>[8x]SRPLSDQEKRKQISVRGLAGVENVTELKKNFNRHLHFTLVKDRNVATPRDYYFALAHTVRDHLVGRWIRTQQHYYEKDPKRIYYLSLEFYMGRTLQNTMVNLALENACDEATYQLGLDMEELEEIEEDAGLGNGGLGRLAACFLDSMATLGLAAYGYGIRYEFGIFNQKICGGWQMEEADDWLRYGNPWEKARPEFTLPVHFYGRVEHTSQGAKWVDTQVVLAMPYDTPVPGYRNNVVNTMRLWSAKAPNDFNLKDFNVGGYIQAVLDRNLAENISRVLYPNDNFFEGKELRLKQEYFVVAATLQDIIRRFKSSKFGCRDPVRTNFDAFPDKVAIQLNDTHPSLAIPELMRVLVDLERLDWDKAWEVTVKTCAYTNHTVLPEALERWPVHLLETLLPRHLQIIYEINQRFLNRVAAAFPGDVDRLRRMSLVEEGAVKRINMAHLCIAGSHAVNGVARIHSEILKKTIFKDFYELEPHKFQNKTNGITPR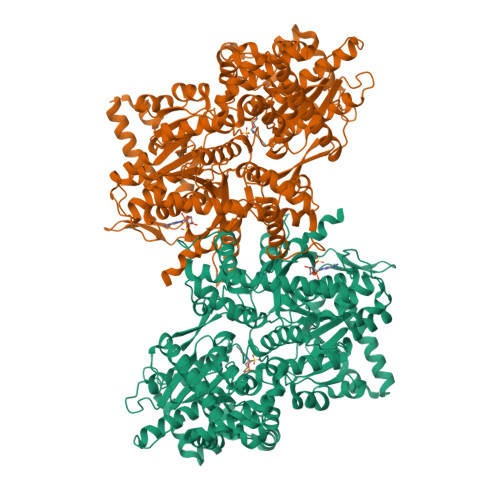RWLVLCNPGLAEIIAERIGEEYISDLDQLRKLLSYVDDEAFIRDVAKVKQENKLKFAAYLEREYKVHINPNSLFDVQVKRIHEYKRQLLNCLHVITLYNRIKKEPNKFVVPRTVMIGGKAAPGYHMAKMIIKLITAIGDVVNHDPVVGDRLRVIFLENYRVSLAEKVIPAADLSEQISTAGTEASGTGNMKFMLNGALTIGTMDGANVEMAEEAGEENFFIFGMRVEDVDRLDQRGYNAQEYYDRIPELRQIIEQLSSGFFSPKQPDLFKDIVNMLMHHDRFKVFADYEEYVKCQERVSALYKNPREWTRMVIRNIATSGKFSSDRTIAQYAREIWGVEPSRQRLPAPDEKIP>[9x]GTMTFQFRNPNFGGNPNNGAFLLNSAQAQNSYKDPSYNDDFGIETPSALDNFTQAIQSQILGGLLSNINT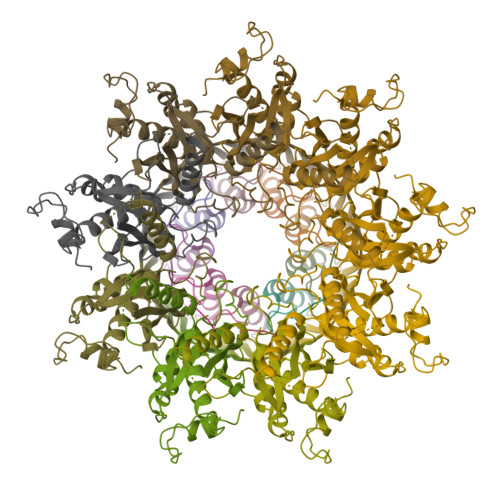GKPGRMVTNDYIVDIANRDGQLQLNVTDRKTGQTSTIQVSGLQNNSTDFHHHHHH;>[9x]CLTAPPKEAARPTLMPRAQSYKDLTHLPAPTGKIFVSVYNIQDETGQFKPYPASNFSTAVPQSATAMLVTALKDSRWFIPLERQGLQNLLNERKIIRAAQENGTVAINNRIPLQSLTAANIMVEGSIIGYESNVKSGGVGARYFGIGADTQYQLDQIAVNLRVVNVSTGEILSSVNTSKTILSYEVQAGVFRFIDYQRLLEGEVGYTSNEPVMLCLMSAIETGVIFLINDGIDRGLWDLQNKAERQNDILVKYRHMSVPPESSAWSHPQFEK>[6x]GMFTCKVNEHITIRLLEPKDAER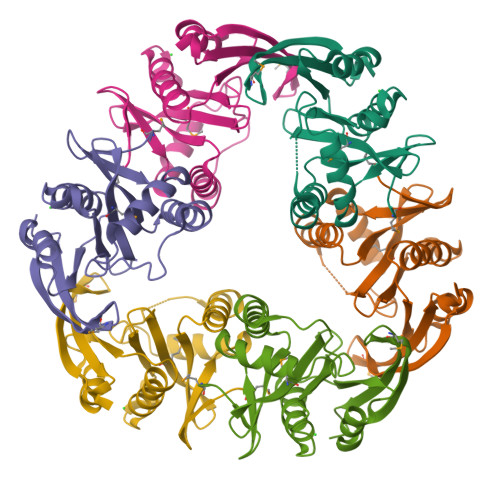LAELIIQNQQRLGKWLFFAENPSSADTYRETIIPDWRRQYADLNGIEAGLLYDGSLCGMISLHNLDQVNRKAEIGYWIAKEFEGKGIITAACRKLITYAFEELELNRVAICAAVGNEKSRAVPERIGFLEEGKARDGLYVNGMHHDLVYYSLLKREWEGEK> GSHMASNNRLFVGSIPKSKTKEQILEEFSKVTEGLTDVILYHQPDDKKKNRGFCFLEYEDHKTAAQARRRLMSGKVKVWGNVGTVEWADPIEDPDPEVMAKVKVLFVRNLANTVTEEILEKAFSQ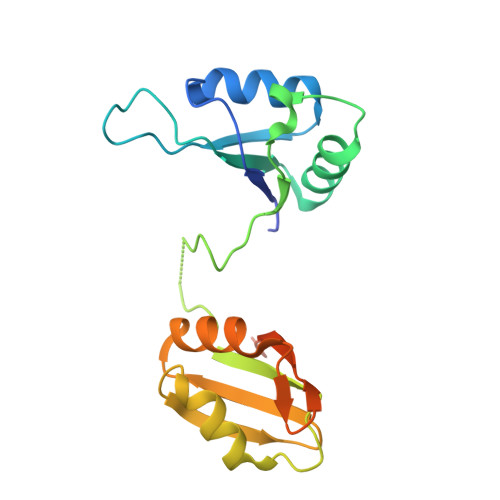FGKLERVKKLKDYAFIHFDERDGAVKAMEEMNGKDLEGENIEIVFAKPPDQKRKERKAQRQAAKNQMY> GHMGQSPDAPIADTPGEQQEINLYSSRHYNTDNELYAKFTAETGIKVNLIEGKADELLERIKSEGANSPADVLLTVDLARLWRAEEDGIFQPVQSEILETNVPEYLRSPDGMWFGFTKRARVIMYNKGKVKPEELSTYEELADPKWKGRVIIRSSSNEYNQSLVASLVVADGEESTLAWAKGFVSNFAREPQGNDTAQIEAVSSGEADLTLANTYY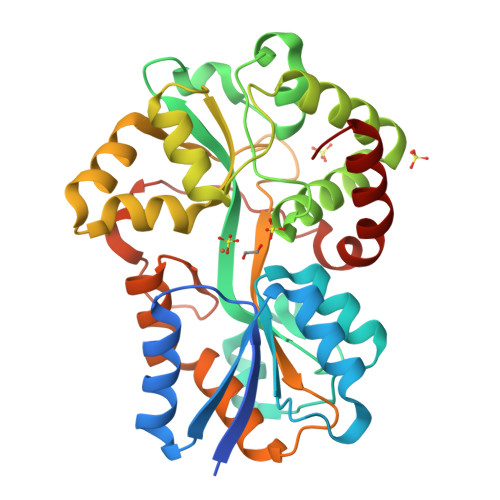MGRLLESEDPAQKAIAENVGVFFPNQEGRGTHVNVSGVGVVKTAPNREGAVKFIEFLVSEPAQAFLAQNNYEYPVLAGVPLNKSVASFGEFKSDTTSLDKLGPALAPATKIMNEAGWK>[3x]MKLPVREFDAVVIGAGGAGMRAALQISQSGQTCALLSKVFPTRSHTVSAQGGITVALGNTHEDNWEWHMYDTVKGSDYIGDQDAIEYMCKTGPEAILELEHMGLPFSRLDDGRIYQRPFGGQSKNFGGEQAARTAAAADRTGHALLHTLYQQNLKNHTTIFSEWYALDLVKNQDGAVVGCTALCIETGEVVYFKARATVLATGGAGRIYQSTTNAHINTGDGVGMAIRAGVPVQDMEMWQFHPTGIAGAGVLVTEGCRGEGGYLLNKHGERFMERYAPNAKDLAGRDVVARSIMIEIREGRGCDGPWGPHAKLKLDHLGKEVLESRLPGILELSRTFAHVDPVKEPIPVIPTCHYMMGGIPTKVTGQALTVNEKGEDVVVPGLFAVGEIACVSVHGANRLGGNSLLDLVVFGRAAGLHLQESIAEQGALRDASESDVEASLDRLNRWNNNRNGEDPVAIRKALQECMQHNFSVFREGDAMAKGLEQLKVIRERLKNARLDDTSSEFNTQRVECLELDNLMETAYATAVSANFRTESRGAHSRFDFPDRDDENWLCHSLYLPESESMTRRSVNMEPKLRPAFPPKIRTY;>[3x]MRLEFSIYRYNPDVDDAPRMQDYTLEADEGRDMMLLDALIQLKEKDPSLSFRRSCREGVCGSDGLNMNGKNGLACITPISALNQPGKKIVIRPLPGLPVIRDLVVDMGQFYAQYEKIKPYLLNNGQNPPAREHLQMPEQREKLDGLYECILCACCSTSCPSFWWNPDKFIGPAGLLAAYRFLIDSRDTETDSRLDGLSDAFSVFRCHSIMNCVSVCPKGLNPTRAIG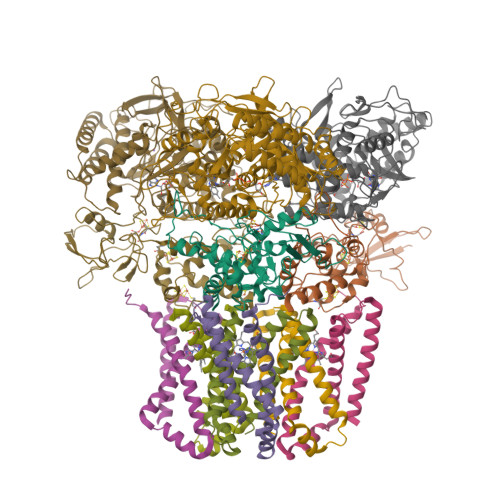HIKSMLLQRNA;>MIRNVKKQRPVNLDLQTIRFPITAIASILHRVSGVITFVAVGILLWLLGTSLSSPEGFEQASAIMGSFFVKFIMWGILTALAYHVVVGIRHMMMDFGYLEETFEAGKRSAKISFVITVVLSLLAGVLVW[3x];>[3x]MVSNASALGRNGVHDFILVRATAIVLTLYIIYMVGFFATSGELTYEVWIGFFASAFTKVFTLLALFSILIHAWIGMWQVLTDYVKPLALRLMLQLVIVVALVVYVIYGFVVVWGV> GPANECISVKGRIYSILKQIGSGGSSKVFQVLNEKKQIYAIKYVNLEEADNQTLDSYRNEIAYLNKLQQHSDKIIRLYDYEITDQYIYMVMECGNIDLNSWLKKKKSIDPWERKSYW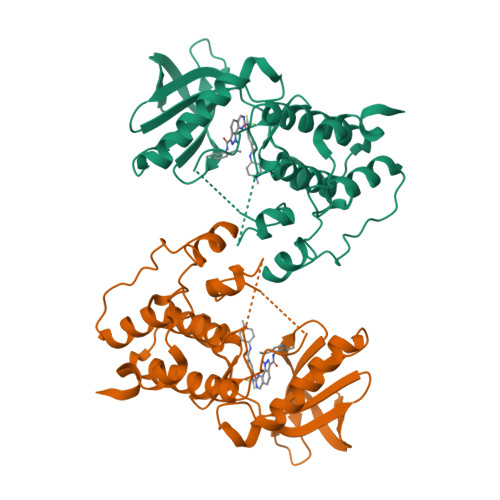KNMLEAVHTIHQHGIVHSDLKPANFLIVDGMLKLIDFGIANQMQPDTTSVVKDSQVGTVNYMPPEAIKDMSSSRENGKSKSKISPKSDVWSLGCILYYMTYGKTPFQQIINQISKLHAIIDPNHEIEFPDIPEKDLQDVLKCCLKRDPKQRISIPELLAHPYVQIQTHPVNQMAKGTTEEMKYVLGQLVGLNSPNSILKA> LKLCSPEEFTRLCREKTQEIYPIKEANGRTRKALIICNTEFKHLSLRYGANFDIIGMKGLLEDLGYDVVVKEELTAEGMESEMKDFAALSEHQTSDSTFLVLMSHGTLHGICGTMHSEKTPDVLQYDT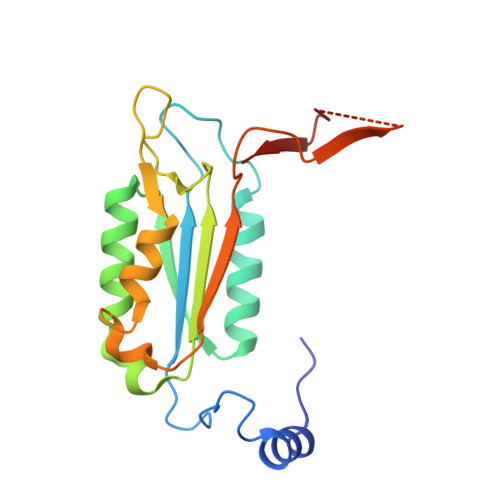IYQIFNNCHCPGLRDKPKVIIVQAARGGNSGEMWIRESSKPQLCRGVDLPRNMEAD> MHHHHHHSSGRENLYFQGRAPQPVVARCKLVLVGDVQCGKTAMLQVLAKDCYPETYVPTVFENYTACLETEEQRVELSLWDTSGSPYYDNVRPLCYSDSDAVLLCFDISRPETVDSALKKWRTEILDYCPSTRVLLIGCKTDLRTDLS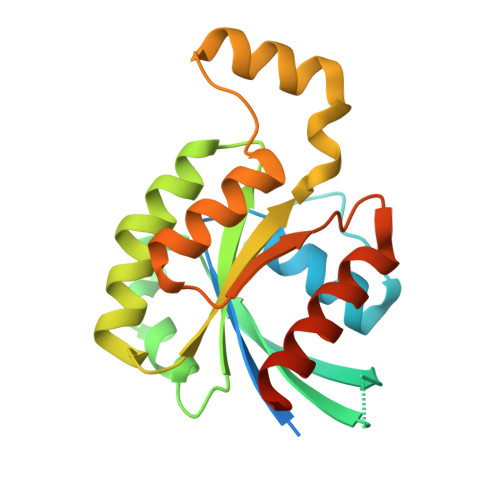TLMELSHQKQAPISYEQGCAIAKQLGAEIYLEGSAFTSEKSIHSIFRTASMLCLNKPSPLPQKSPV>PEIIIGDLQILPDAFVAKKRGTEVELTHREFELLHHLATHTG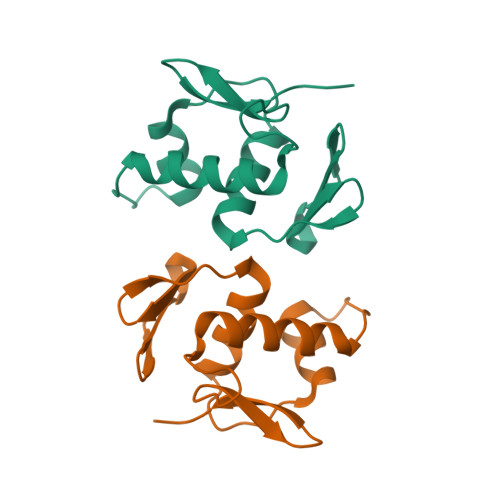QVMTREHLLETVWGYDYFGDVRTVDVTVRRLREKIEDTPSRPEYILTRRGVGYYMKSYD[2x]>GQKKTKFKAADLKGIWQL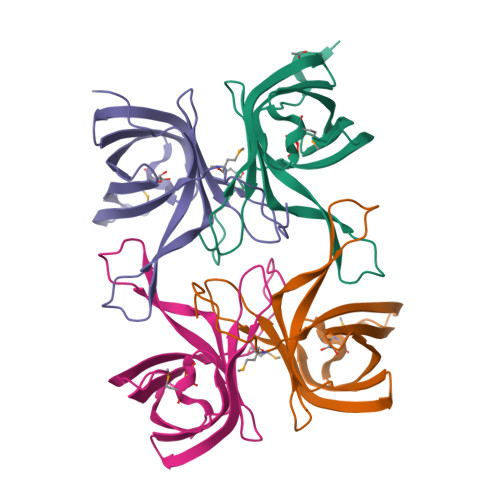CHYVSESPDVPGALKPSNTFKVLSDDGRIVNFTIIPGADAIITGYGTYKQLTDDSYKESIEKNIHLPMLDNQDNILEFEIKDNDYLHLKYFIKSDLNGNELNTWYYETWKRVEMPAKFPEDIVR[8x]> AEST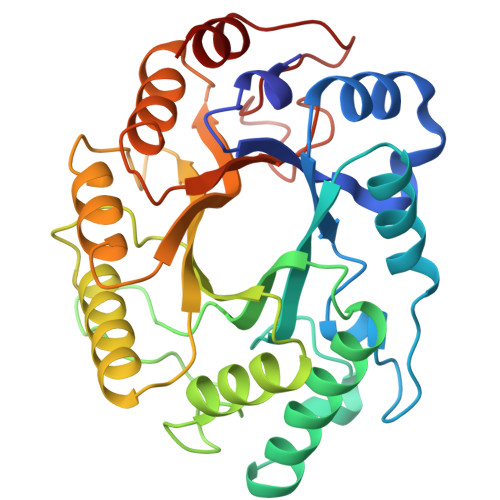LGAAAAQSGRYFGTAIASGRLSDSTYTSIAGREFNMVTAENEMKIDATEPQRGQFNFSSADRVYNWAVQNGKQVRGHTLAWHSQQPGWMQSLSGRPLRQAMIDHINGVMAHYKGKIVQWDVVNEAFADGSSGARRDSNLQRSGNDWIEVAFRTARAADPSAKLCYNDYNVENWTWAKTQAMYNMVRDFKQRGVPIDCVGFQSHFNSGSPYNSNFRTTLQNFAALGVDVAITELDIQGAPASTYANVTNDCLAVSRCLGITVWGVRDSDSWRSEQTPLLFNNDGSKKAAYTAVLDA>MGHHHHHHMMKFINIGYGNMVSAARIITIVSPDSAPIKRIIQDAREKGKLVDATHGRATAAVIITDSDHVILSSVQPETVANRLYGSDDFSEEG[2x]

Bacillus subtilis can form structurally complex biofilms on solid or liquid surfaces, which requires expression of genes for matrix production. The transcription of these genes is activated by regulatory protein RemA, which binds to poorly conserved, repetitive DNA regions but lacks obvious DNA-binding motifs or domains. Here, we present the structure of the RemA homologue from Geobacillus thermodenitrificans, showing a unique octameric ring with the potential to form a 16-meric superstructure. These results, together with further biochemical and in vivo characterization of B. subtilis RemA, suggests that the protein can wrap DNA around its ring-like structure through a LytTR-related domain.

The (His)6-tag present at the N-terminus of RemA did not affect the binding of the wildtype protein to DNA fragments containing PepsA in the EMSAs, because a tag-free variant of (Gt)RemA showed the same DNA-binding behavior as its His-tagged counterpart. These findings show that DNA-binding by RemA involves the arginines 50 and 51. To investigate whether the variation of these residues impacts the structure of (RemA), we aimed at crystallizing the (Gt)RemA-R50A and -R51A variants. Unfortunately, both variants did not crystallize, likely due to the lack of the arginines 50 and 51, which are relevant to establish crystal contacts involving the sulfate ions. Superimposition of wildtype (RemA)8 and (RemA-R51A/R53A)8 shows that both structures are identical (r.m.s.d. of 0.3 Å over 600 Cα-atoms) and the positions of R51 and R53 overlap with the varied alanines in the RemA-R51A/R53A structure. This analysis shows that variations of these arginines does neither impact the quaternary nor the tertiary structure of RemA but impairs DNA-binding.>[16x]ARGAATRARQKQRASLETMDKAVQRFRLQNPDLDSEALLTLPLLQLVQKLQSGELSPEAVFFTYLGKAWEVNKGTNCVTSYLTDCETQLSQAPRQGLLYGVPVSLKECFSYKGHDSTLGLSLNEGMPSESDCVVVQVLKLQGAVPFVHTNVPQSMLSFDCSNPLFGQTMNPWKSSKSPGGSSGGEGALIGSGGSPLGLGTDIGGSIRFPSAFCGICGLKPTGNRLSKSGLKGCVYGQTAVQLSLGPMARDVESLALCLKALLCEHLFTLDPTVPPLPFREEVYRSSRPLRVGYYETDNYTMPSPAMRRALIETKQRLEAAGHTLIPFLPNNIPYALEVLSAGGLFSDGGRSFLQNFKGDFVDPCLGDLILILRLPSWFKRLLSLLLKPLFPRLAAFLNSMRPRSAEKLWKLQHEIEMYRQS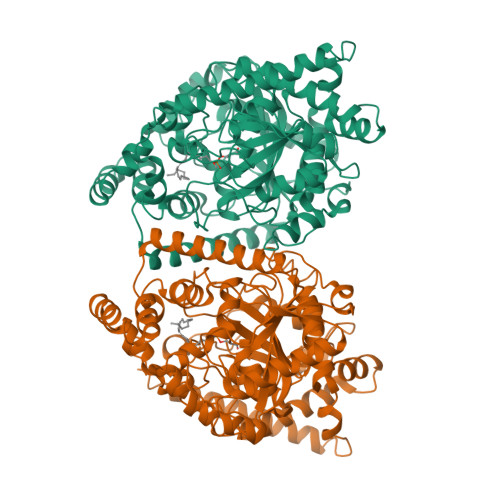VIAQWKAMNLDVLLTPMLGPALDLNTPGRATGAISYTVLYNCLDFPAGVVPVTTVTAEDDAQMELYKGYFGDIWDIILKKAMKNSVGLPVAVQCVALPWQEELCLRFMREVEQLMT>GGAGGGGAACUUCUAUCUGGUGAUAGACGGGAACUCUAAAUUCCUUGAAAUGCCUCGCCGCAUUGGGUUCGAUUCCCUUCCCCUCCGCCA[3x]

A search of metagenomic sequences revealed uniquely structured tRNAs (allo-tRNAs) containing recognition elements that resembled tRNASec but with a 12 bp acceptor domain (acceptor and T-stem combined) for proper recognition by EF-Tu. Specifically, tRNAUTu1 was found to be a serine isoacceptor with a 9/3 (acceptor/T-stem bp) structure that allowed EF-Tu driven Sec incorporation. Here, we investigated the suitability of an allo-tRNA, tRNAUTu1, for translation by E. coli ribosomes, and demonstrate the importance of global tRNA structure for efficient translation. tRNAUTu1 is used for site-specific insertion of Sec by harnessing EF-Tu to avoid constraints on natural Sec translation. Implementing cryo-EM, we visualized tRNAUTu1 in complex with the E. coli ribosome to pinpoint the structural feature in tRNAUTu1 hindering translation.

To visualize structures and orientations of tRNAUTu1 in the ribosome, we used single-particle cryo-EM on samples of tRNAUTu1 in complex with the E. coli 70S ribosome. The complex was prepared by programming tRNAUTu1 to bind in all ribosomal sites using an mRNA containing three tandem UAG codons. The global resolution of the triple tRNAUTu1 and ribosome complex is 2.6 Å, allowing atomic-level modeling. The distance and angles between the acceptor stem and anticodon stem are conserved, allowing tRNAUTu1 to reach into both the peptidyl transferase center and the decoding center, essential for tRNA function. Overall, the structural features of tRNAUTu1 in the ribosomal A site led to an 8.7 Å shift of the variable loop as compared to tRNASec. When tRNAUTu1 is bound in the P site, both the acceptor stem and the anticodon stem conformations are conserved, allowing them to reach into both the peptidyl transferase center and the decoding center. The variable loop of tRNAUTu1 is shifted by 10 Å compared with its conformation in the A site. This movement creates a 17° rotation of the variable loop upwards towards the ribosome to avoid a clash with the A-site finger (ASF), a functional attenuator for translocation. The additional constraint on tRNAUTu1 variable loop orientation imposed by the ribosomal scaffold could raise the energetic barrier for tRNAUTu1 translocation, and steric clash could lead to ribosome disassembly, as observed by single-molecule FRET. The central loop of tRNAUTu1 does not interact with any of the stems, but A45 base paring with C8 was identified as a key stabilizing element of the central loop.> MSTQLASNIYAPLYAPFFGFAGCAAAMVLSCLGAAIGTAKSGIGIAGIGTFKPELIMKSLIPVVMSGILAIYGLVVAVLIAGNLSPTEDYTLFNGFMHLSCGLCVGFACLSSGYAIGMVGDV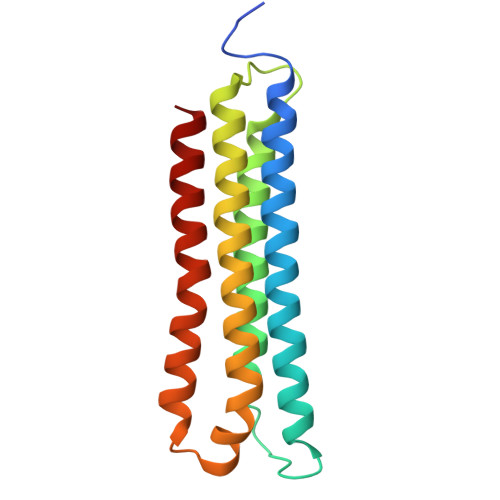GVRKYMHQPRLFVGIVLILIFSEVLGLYGMIVALILNTRGSE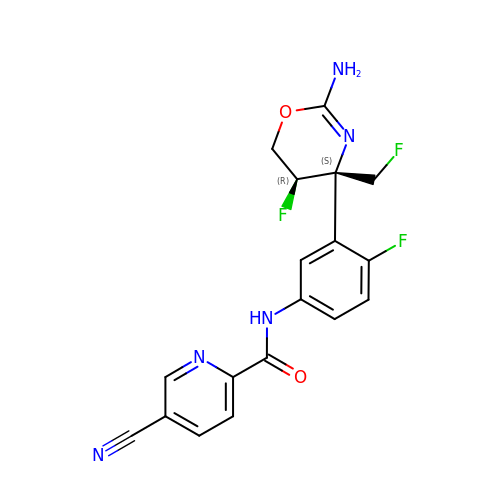N-{3-[(4S,5R)-2-amino-5-fluoro-4-(fluoromethyl)-5,6-dihydro-4H-1,3-oxazin-4-yl]-4-fluorophenyl}-5-cyanopyridine-2-carboxamide | C18 H14 F3 N5 O2 | MMPPCMJOPZGPPA-MAUKXSAKSA-N3-[(carboxymethyl)sulfanyl]pyridine-2-carboxylic acid | C8 H7 N O4 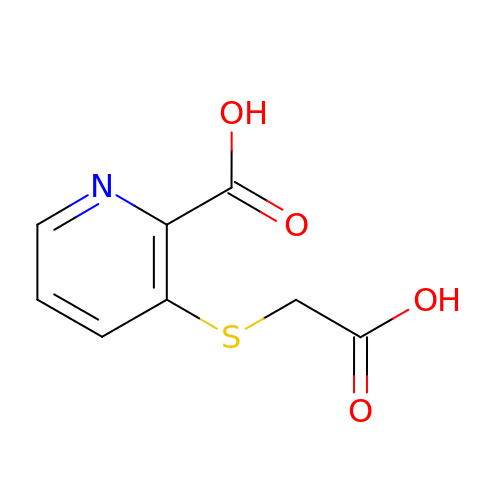S | LQCDNBQBBOQQIK-UHFFFAOYSA-N> GEIEFIESSKDAGFPVINTPSKTKLEPSVFHQVFEGNKEPAVLRSGDPRLKANF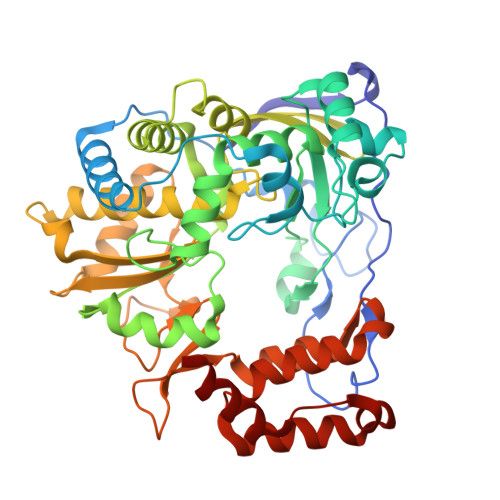EEAIFSKYIGNVNTHVDEYMLEAVDHYAGQLATLDISTEPMKLEDAVYGTEGLEALDLTTSAGYPYVALGIKKRDILSKKTKDLTKLKECMDKYGLNLPMVTYVKDELRSIEKVAKGKSRLIEASSLNDSVAMRQTFGNLYKTFHLNPGVVTGSAVGCDPDLFWSKIPVMLDGHLIAFDYSGYDASLSPVWFACLKMILEKLGYTHKETNYIDYLCNSHHLYRDKHYFVRGGMPSGCSGTSIFNSMINNIIIRTLMLKVYKGIDLDQFRMIAYGDDVIASYPWPIDASLLVEAGKGYGLIMTPADKGECFNEVTWTNVTFLKRYFRADEQYPFLVHPVMPMKDIHESIRWTKDPKNTQDHVRSLCLLAWHNGEHEYEEFIRKIRSVPVGRCLTLPAFSTLRRKWLDSF> GAMAWALKTINPGLFEEPAKTSEASKSNGQSVSL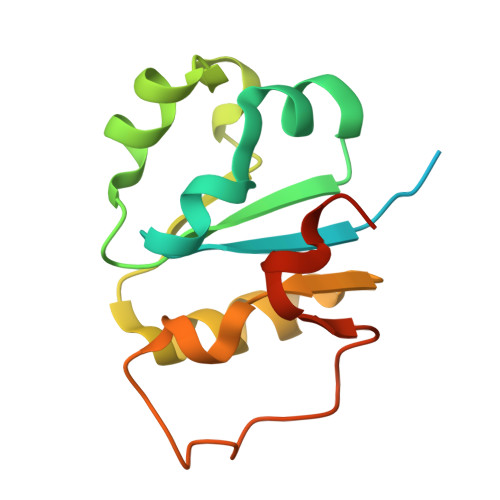VLTQKDLDFFSAAYLNEYPNLTVILHPSVDKSEFLSRFNVQRNSHQVIQVRTEESIFHVLKQLSSNINLITLGNLEMSANEVETFHLDKFLTNVHEVDRINDYI> MEGVYTVTVYPGDPAFEIQDSLPQKIWPMLYLHQQRWLPSYGPWHIRFTSSAMQLRNFPRSLRGQANFQNSMSLKLITALTDVISRISLDFYSDLRHLSDTMSALCLIAAYYSEKNQTPLPTNLPELLGNITAKVTLLVRDLKRAAANKGFNFNRNSSSLLPAQGGLYSNDFFQEHALYSLFRTAGMLASSSSPEYPRADSVLAITAAVFGDNIPPFAAYQWNLRSGLKALESLILLFLLLDVNVPATSNKRLHLEALLGESYSKGSRPPARRTGPLDAGGSVFSFLMENYLVPTLLHRPTTNMSALFPGLYLLQLEFSSGASTPHAIHLTDVKFRDIFNILVQSNVFQDSQELIRAKQSLRVSCETGSGNLLESLSPGTTMRDIIRKEFMAQDVYDYV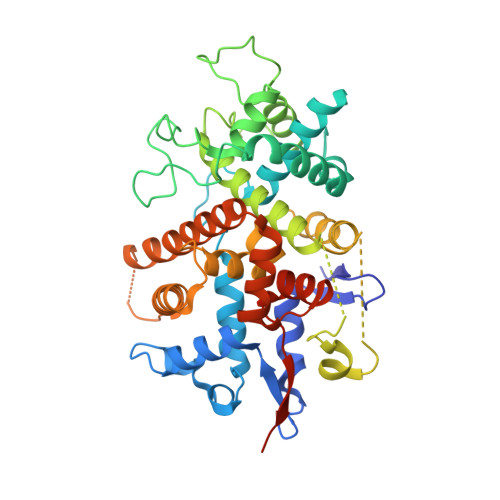YFCVLGALPVTVAVVPAAALEHHHHHHHHH Paraplegin is an m-AAA protease of the mitochondrial inner membrane that is linked to hereditary spastic paraplegias. Human paraplegin (SPG7) is a mitochondrial membrane-associated AAA-domain containing metalloprotease consisting of three homology domains: The N-terminal FtsH-extracellular domain, which is found in membrane-bound ATP-dependent proteases; the intermediate AAA-domain; and the C-terminal metallopeptidase M41 domain. The protein is believed to form a hexamer that uses ATPase-driven conformational changes in its AAA-domain to deliver substrate peptides to its protease domain. Paraplegin is implicated in the degradation of proteins that come out misfolded after transport across the mitochondrial membranes, and in cleavage of mitochondrial targeting sequences.

We purified recombinant human paraplegin including residues 305–565 (corresponding to the ATPase domain) in the absence of excess nucleotide. We determined the crystal structure of this protein to a resolution of 2.2 Å. The protein crystallized with one monomer in the asymmetric unit, and ADP was bound in the nucleotide binding site. The structure shows the typical AAA+ domain consisting of a five-stranded parallel β-sheet flanked by two α-helices on each side, together with a carboxy-terminal bundle of four antiparallel α-helices (Figure 3 and Supplementary Datapack S1). The nucleotide binding pocket is located at the interface between the β-sheet and the α-helical bundle. Despite high concentrations of ATP and Mg2+ during crystallization, ADP was clearly seen in the electron density, and as in previously determined FtsH structures, density for a magnesium ion was not observed. The conserved P-loop in the Walker A motif (GxxGxGK(T/S); residues Gly 350 – Thr 356), is central in binding the β–phosphate of ADP through hydrogen bonding interactions with the backbone nitrogens of residues 352 – 356, the Lys 355 and Thr 356 side chains, and a water molecule. The adenine base is stacked between the hydrophobic side chains of Leu 357 and Ile 448, and hydrogen bonds with the His 492 side chain, the backbone amide and oxygen of Ala 312, and two water molecules. The pore loop of the paraplegin AAA-domain contains the sequence Ile 382 – Gly 384 (IGG), and alignment of our structure with the FtsH hexamer show that the Ile 382 side chains of paraplegin line the central pore in a similar fashion as the Phe 229 side chains of FtsH. Most of the known disease mutations in the SPG7 gene lead to premature termination or map to the metallopeptidase domain. Some mutations, however, have been identified in the AAA+ domain, and surprisingly, they all map to the C-terminal α-helical bundle (Figure 1B and Supplementary Datapack S1).

> MGVSFKDVAGMHEAKLEVREFVDYLKSPERFLQLGAKVPKGALLLGPPGCGKTLLAKAVATEAQVPFLAMAGAEFVEVIGGLGAARVRSLFKEARARAPCIVYIDEIDAVGKKRSTTMSGFSNTEEEQTLNQLLVEMDGMGTTDHVIVLASTNRADILDGALMRPGRLDRHVFIDLPTLQERREIFEQHLKSLKLTQSSTFYSQRLAELTPGFSGADIANICNEAALHAAREGHTSVHTLNFEYAVERVLAGTAKKSKILSK>MNHKVHHHHHHIEGRHMPDDLNAVVTELDKEGVKYKISPDGRTIYVPENVARELRLKLAAKGVPRKGIVGYELFDKSGIVLSRFQQLVNFKRAIEGELAKTIMSLDCVEFARVHIVLPEKSLFIREEEEAKASVF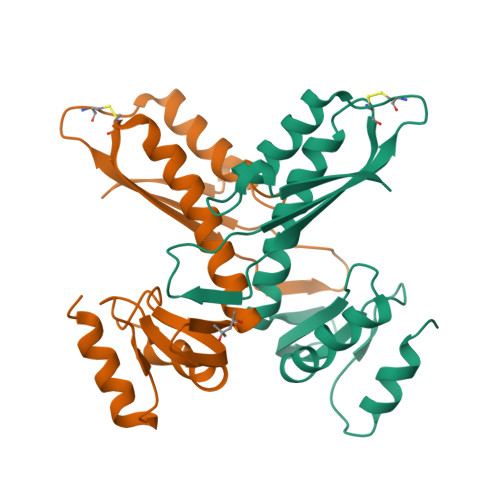LKLKPGCELTPEQVKAIRNLVSGSVENLKPSQVVVVDD[2x]>[2x]MQQKSDNVVSHYVFEAPVRIWHWLTVLCMAVLMVTGYFIGKPLPSVSGEATYLFYMGYIRLIHFSAGMVFTVVLLMRIYWAFVGNRYSRELFIVPVWRKSWWQGVWYEIRWYLFLAKRPSADIGHNPIAQAAMFGYFLMSVFMIITGFALYSEHSQYAIFAPFRYVVEFFYWTGGNSMDIHSWHRLGMWLIGAFVIGHVYMALREDIMSDDTVISTMVNGYRSHKFGKISNKERS;>[4x]MSTQYETQGYTINNAGRRLVVDPITRIEGHMRCEVNINDQNVITNAVSCGTMFRGLEIILQGRDPRDAWAFVERICGVCTGVHALASVYAIEDAIGIKVPDNANIIRNIMLATLWCHDHLVHFYQLAGMDWIDVLDALKADPRKTSELAQSLSSWPKSSPGYFFDVQNRLKKFVEGGQLGIFRNGYWGHPQYKLPPEANLMGFAHYLEALDFQREIVKIHAVFGGKNPHPNWIVGGMPCAINIDESGAVGAVNMERLNLV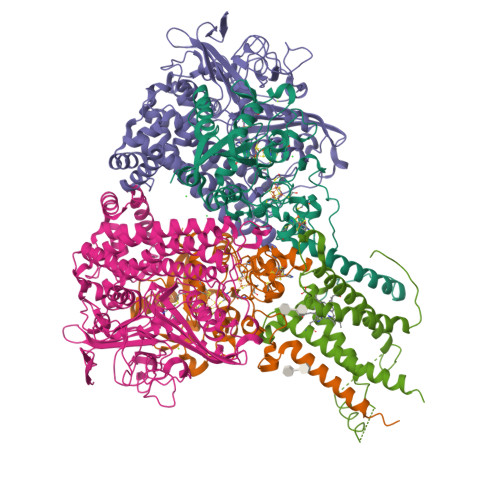QSIITRTADFINNVMIPDALAIGQFNKPWSEIGTGLSDKCVLSYGAFPDIANDFGEKSLLMPGGAVINGDFNNVLPVDLVDPQQVQEFVDHAWYRYPNDQVGRHPFDGITDPWYNPGDVKGSDTNIQQLNEQERYSWIKAPRWRGNAMEVGPLARTLIAYHKGDAATVESVDRMMSALNLPLSGIQSTLGRILCRAHEAQWAAGKLQYFFDKLMTNLKNGNLATASTEKWEPATWPTECRGVGFTEAPRGALGHWAAIRDGKIDLYQCVVPTTWNASPRDPKGQIGAYEAALMNTKMAIPEQPLEILRTLHSFDPCLACSTH;>LENKPRIPVVWIHGLECTCCTESFIRSAHPLAKDVILSLISLDYDDTLMAAAGTQAEEVFEDIITQYNGKYILAVEGNPPLGEQGMFCISSGRPFIEKLKRAAAGASAIIAWGTCASWGCVQAARPNPTQATPIDKVITDKPIIKVPGCPPIPDVMSAIITYMVTFDRLPDVDRMGRPLMFYGQRIHDKCYRRAHFDAGEFVQSWDDDAARKGYCLYKMGCKGPTTYNACSSTRWNDGVSFCIQSGHGCLGCAENGFWDRGSFYSRVVDIPQMGTHSTADTVGLTALGVVAAAVGVHAVASAVDQRRRHNQQPTETEHQPGNEDKQARSHHHHHH[4x]7-{3-(aminomethyl)-4-[(1,3-thiazol-4-yl)methoxy]phenyl}-4-methylquinolin-2-amine | C21 H20 N4 O S | 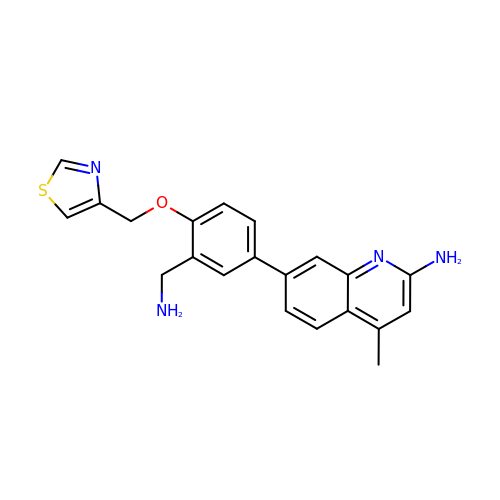QMLWVSKDYLAYRJ-UHFFFAOYSA-N>[2x]HMTDLKASSLRALKLMDLTTLNDDDTDEKVIALCHQAKTPVG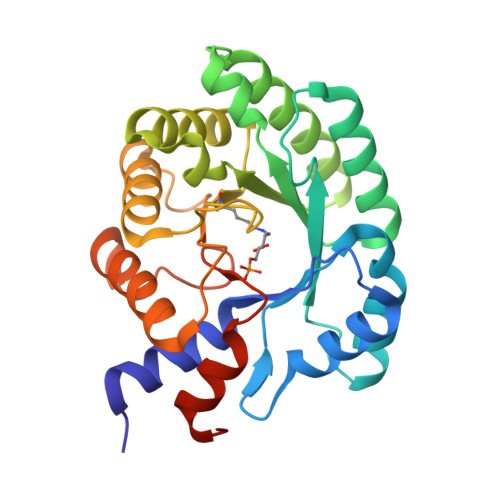NTAAICIYPRFIPIARKTLKEQGTPEIRIATVTNFPHGNDDIDIALAETRAAIAYGADEVDVVFPYRALMAGNEQVGFDLVKACKEACAAANVLLKVIIETGELKDEALIRKASEISIKAGADFIKTSTGKVAVNATPESARIMMEVIRDMGVEKTVGFLPAGGVRTAEDAQKYLAIADELFGADWADARHYRFGASSLLASLLKALGHGDGKSASSY> GSMPKPINVRVTTMDAELEFAIQPNTTGKQLFDQVVKTVGLREVWFFGLQYVDSKGYSTWLKLNKKVTQQDVKKENPLQFKFRAKFFPEDVSEELIQEITQRLFFLQVKEAILNDEIYCPPETAVLLASYAVQAKYGDYNKEIHKPGYLANDRLLPQRVLEQHKLTKEQWEERIQNWHEEHRGMLREDSMMEYLKIAQDLEMYGVNYFEIKNKKGTELWLGVDALGLNIYEHDDKLTPKIGFPWSEIRNISFNDKKFVIKPIDKKAPDFVFY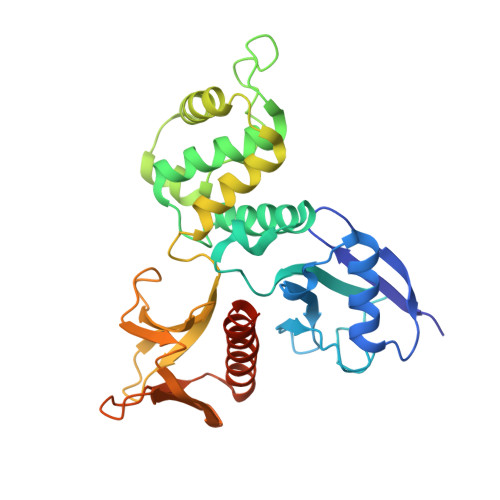APRLRINKRILALCMGNHELYMRRRKPDTIEVQQMKAQAR>[2x]SENDVIELDDVANLMFYGEGEVGDNHQKFMLIFDTGSANLWVPSKKCNSIGCSTKHLYDSSKSKSYEKDGTKVEITYGSGTVRGFFSKDLVTLGYLSLPYKFIEVTDTDDLEPLYTAAEFDGILGLGWKDLSIGSIDPIVVELKNQNKIDQALFTFYLPVHDKHSGYLTIGGIEEKFYEGELTYEKLNHDLFWQVDLDVNFGKTSMEKANVIVDSGTSTI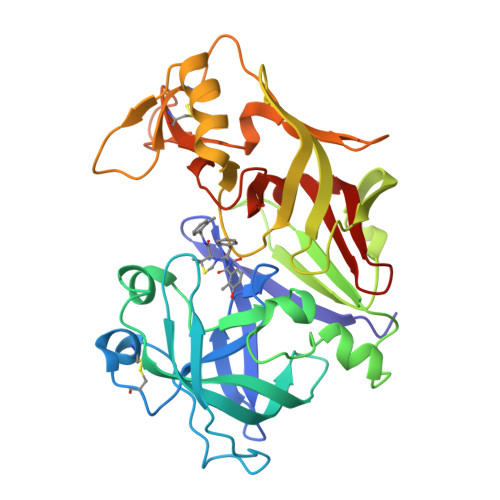TAPTSFINKFFKDLNVIKVPFLPFYITTCNNKDMPTLEFKSANNTYTLEPEYYMEPLLDIDDTLCMLYILPVDIDKNTFILGDPFMRKYFTVFDYDKESIGFAVAKN>[2x]HHHHHHGSSQLLPAPLTNDPTAI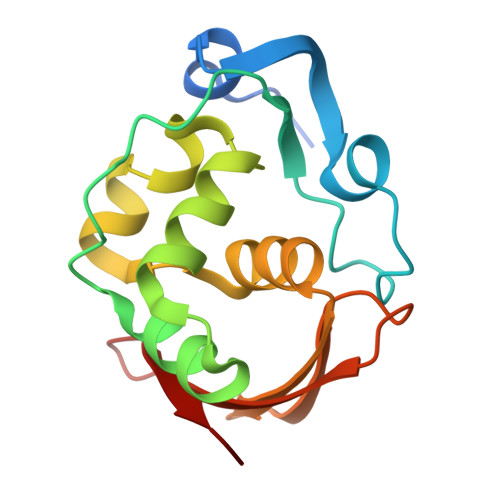GPVLPFEELHPRRYPENTATFLTRLRSLPSNHLPQPTLNCLLSAVSDQTKVSEEHLWESLQTILPDSQLSNEETNTLGLSTEHLTALAHLYNFQATVYSDRGPILFGPSDTIKRIDITHTTGPPSHFSPGK[(2R,3S,4R,5R,6R)-5-acetamido-6-[[[(2R,3S,4R,5R)-5-[2,4-bis(oxidanylidene)pyrimidin-1-yl]-3,4-bis(oxidanyl)oxolan-2-yl]methoxy-oxidanyl-phosphoryl]oxy-oxidanyl-phosphoryl]oxy-3,4-bis(oxidanyl)oxan-2-yl]methylimino-azanylidene-azanium | C17 H27 N6 O16 P2 | 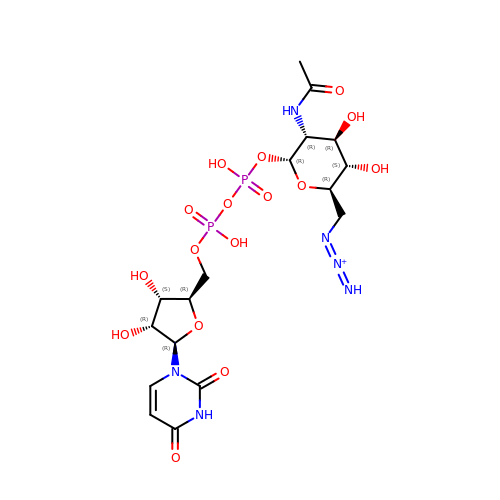JRORMXITLCSMOP-CFRASDGPSA-O>[2x]MVMKQTKQTNILAGAAVIKVLEAWGVDHLYGIPGGSINSIMDALSAERDRIHYIQVRHEEVGAMAAAADAKLTGKIGVCFGSAGPGGTHLMNGLYDAREDHVPVLALIGQFGTTGMNMDTFQEMNENPIYADVADYNVTAVNAATLPHVIDEAIRRAYAHQGVAVVQIPVDLPWQQIPAEDWYASANSYQTPLLPEPDVQAVTRLTQTLLAAERPLIYYGIGARKAGKELEQLSKTLKIPLMSTYPAKGIVADRYPAYLGSANRVAQKPANEALAQADVVLFVGNNY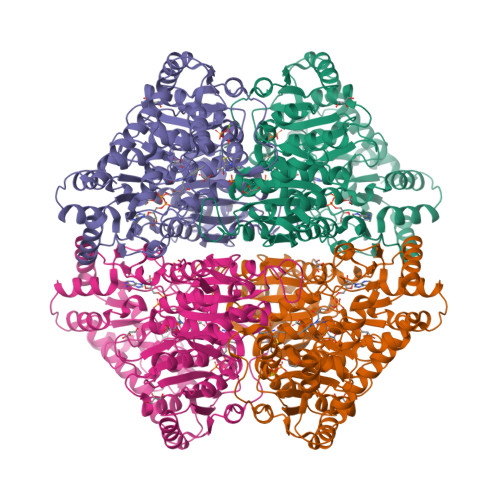PFAEVSKAFKNTRYFLQIDIDPAKLGKRHKTDIAVLADAQKTLAAILAQVSERESTPWWQANLANVKNWRAYLASLEDKQEGPLQAYQVLRAVNKIAEPDAIYSIDVGDINLNANRHLKLTPSNRHITSNLFATMGVGIPGAIAAKLNYPERQVFNLAGDGGASMTMQDLATQVQYHLPVINVVFTNCQYGFIKDEQEDTNQNDFIGVEFNDIDFSKIADGVHMQAFRVNKIEQLPDVFEQAKAIAQHEPVLIDAVITGDRPLPAEKLRLDSAMSSAADIEAFKQRYEAQDLQPLSTYLKQFGLDDLQHQIGQGGF>MSDEKVVSIGAAPLSAKEKLDLYCEGLADGLNKTQAYVAAGFSPNHAQRNVAAYHRKHSEYINAFISERIGSHVPMALRVIVSIAEDPNEKGGIRLKAAQDILDRGGFGAKQKVELTTKNVEDMSAEDLMNEVRRILDEEPDLAKVLSFPTA[9x]

The genome packaging motor of tailed bacteriophages and herpesviruses is a powerful nanomachine built by several copies of a large (TerL) and a small (TerS) terminase subunit. In contrast, TerS is a DNA recognition subunit that binds packaging initiation sites (referred to as pac or cos) in preparation for genome packaging. TerS also stimulates the ATPase activity of TerL, while repressing the large terminase nuclease activity. Thus, three related small terminase subunits from Pseudomonas phages PaP3, NV1 and LUZ24 are polymorphic in solution but adopt a nonameric quaternary structure in the high affinity heparin-binding conformation.

PaP3 TerS crystals diffracted to ∼3 Å resolution with one nonamer in the asymmetric unit (AU). An initial molecular replacement (MR) solution was gradually improved and entirely rebuilt, yielding a complete atomic model of PaP3 TerS currently refined to an Rwork/Rfree of 25.0/27.4%, at 3.0 Å resolution. PaP3 TerS folds into a hollow nonameric ring of mixed α/β structure that resembles a mushroom. The quaternary structure of TerS consists of an apical gear-like ring ∼105 Å in diameter sitting onto a 9-stranded β-barrel ∼50 Å in height, similar to that found in β-porins. Unlike P22, PaP3 TerS lacks a ‘dome-domain’ and is pronouncedly asymmetric. The RMSD between subunits varies between 1.23 Å for chains a-h, the most similar and 1.67 Å, for chains a-i, the most dissimilar. This asymmetry is generated by an uneven pattern of lateral contacts between neighboring protomers. Three pairs of contacting subunits (labeled as i:a) make a close-distance (e.g. 2.5–3.5 Å) salt bridge between R56 and D21 projecting from juxtaposed protomers. The crystal structures of PaP3 and NV1 TerSs presented in this paper revealed a solvent-filled channel of 9.7–15 Å diameter. This channel is too small to accommodate dsDNA, ruling out the viral genome threads through the central channel of TerS during packaging. We demonstrate PaP3 TerS binds DNA through a highly dynamic N-terminal helix-turn-helix (HTH)-motif that adopts a different conformation in solution versus in crystal. After electrophoretic separation, both free DNA and TerS:DNA complexes were visualized using the fluorescence signal of Cy3 and quantified, which revealed PaP3 TerS binds the cos sequence with significantly higher affinity than scrambled DNA. Mutations in the HTH helix α1 (DM-TerS) reduced binding to cos (Figure 6C- and D) by over 70%, confirming this region of the protein is responsible for DNA-binding activity in vitro.16,17-dimethoxy-21-(4-pyridin-4-ylbutyl)-5,7-dioxa-13$l^{4}-azapentacyclo[11.8.0.0^{2,10}.0^{4,8}.0^{15,20}]henicosa-1(21),2(10),3,8,13,15,17,19-octaene 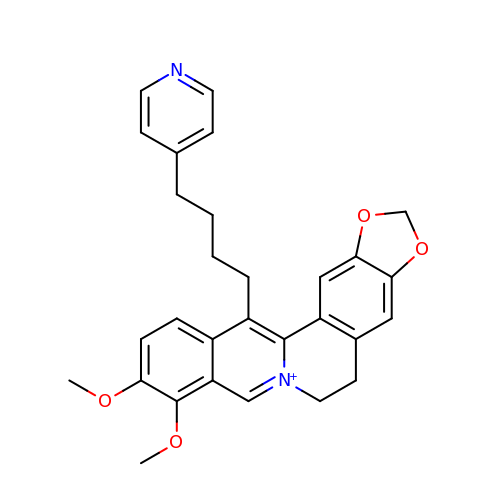| C29 H29 N2 O4 | YAGGXYGFEKMOOG-UHFFFAOYSA-N> ESRYKDNRPLNILGIDISKMELGRYNLFEVSIFLQGSYLNPFDPQEIDVEGIFEDQYGNQYRVPGFFYQEYKRELKNDYEYLVPVGDPYFKIRFSPINIGSYKFFIKVKDKTGREVSSDKYTIYVKESEKPGYIRVSEKNWRYFKFDNGRQFLPIGANICWATSKGTYDYDVWLPKCAENGGNYFRVWLGPSWATFALERESVKEYDLKNAWKLDYVLNLAEKLNMYIMFCFDSYNELRYQKEGAYPYWEHTPHYEKNGGPL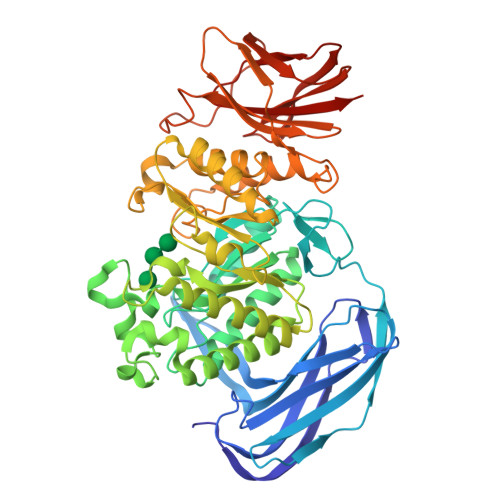KEPKDFWTNNEMIKYYKNKLRYIVARYGYSTNVFAWEFWNQVDIISPTAFVIGEVKKWHEDMAKYLNSIDPWKHLITTSFAFSPGKPEIDSISGLNFVQTHIYKSNRYIDALLSLIAYKEKYRKPHLVGEFGLDAGGNDLWVDPNGYVIHNAIWTTILSGASGTAMSWWWDNHIHPNNLYFHYRALADFVKDINFLEEKFERLTNYKFNVYNREIKVIGLQGKKYILLWLYNAKEAYQYKKDIPNMDSSKFLGSIELLIKPPIKVIYYDTYRGEKIKELDLDKNVIPIIEFERDLAIKIELLGEGE>MLRKLSKFSNKGEVFMGLLEGKRALITGVANERSIAYGIAKSFHRE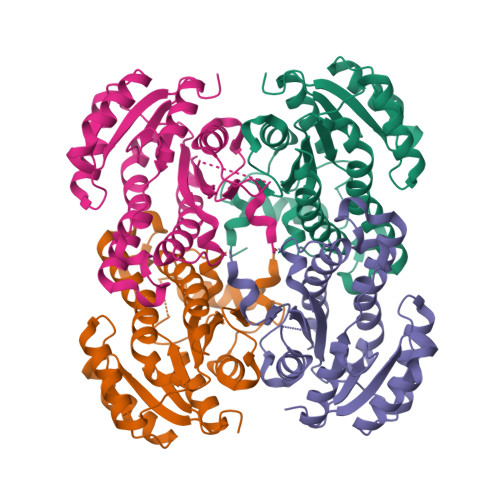GAQLAFTYATPKLEKRVREIAKGFGSDLVVKCDVSLDEDIKNLKKFLEENWGSLDIIVHSIAYAPKEEFKGGVIDTSREGFKIAMDISVYSLIALTRELLPLMEGRNGAIVTLSYYGAEKVVPHYNVMGIAKAALESTVRYLAYDIAKHGHRINAISAGPVKTLAAYSITGFHLLMEHTTKVNPFGKPITIEDVGDTAVFLCSDWARAITGEVVHVDNGYHIMGVFGREEEIKKEVYGD[4x]> MMLSLNNLQNIIYNPVIPFVGTIPDQLD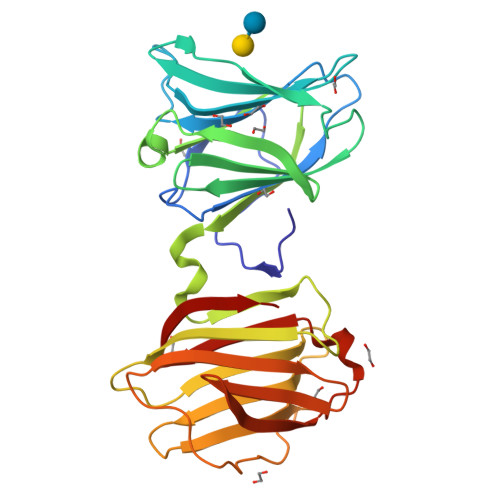PGTLIVIRGHVPSDADRFQVDLQNGSSMKPRADVAFHFNPRFKRAGCIVCNTLINEKWGREEITYDTPFKREKSFEIVIMVLKDKFQVAVNGKHTLLYGHRIGPEKIDTLGIYGKVNIHSIGFSFSSHMRLPFAARLNTPMGPGRTVVVKGEVNANAKSFNVDLLAGKSKDIALHLNPRLNIKAFVRNSFLQESWGEEERNITSFPFSPGMYFEMIIYCDVREFKVAVNGVHSLEYKHRFKELSSIDTLEINGDIHLLEVRSW>[4x]MNSNKELMQRRSQAIPRGVGQIHPIFADRAENCRVWDVEGREYLDFAGGIAVLNTGHLHPKVVAAVEAQLKKLSHTCFQVLAYEPYLELCEIMNQKVPGDFAKKTLLVTTGSEAVENAVKIARAATKRSGTIAFSGAYHGRTHYTLALTGKVNPYSAGMGLMPGHVYRALYPCPLHGISEDDAIAS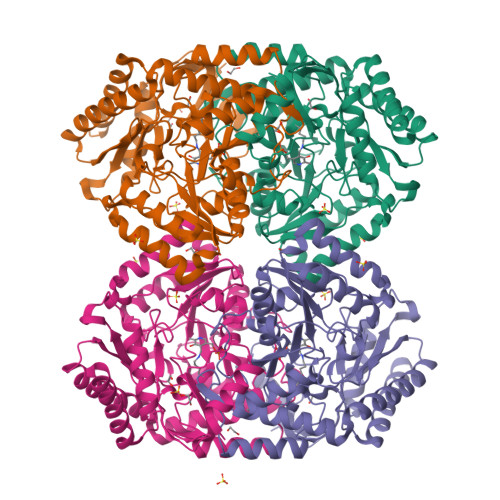IHRIFKNDAAPEDIAAIVIEPVQGEGGFYASSPAFMQRLRALCDEHGIMLIADEVQSGAGRTGTLFAMEQMGVAPDLTTFAKSIAGGFPLAGVTGRAEVMDAVAPGGLGGTYAGNPIACVAALEVLKVFEQENLLQKANDLGQKLKDGLLAIAEKHPEIGDVRGLGAMIAIELFEDGDHNKPDAKLTAEIVARARDKGLILLSCGPYYNVLRILVPLTIEDAQIRQGLEIISQCFDEAKQ> EPREEAGALGPAWDESQLRSYSFPTRPIPRLSQSDPR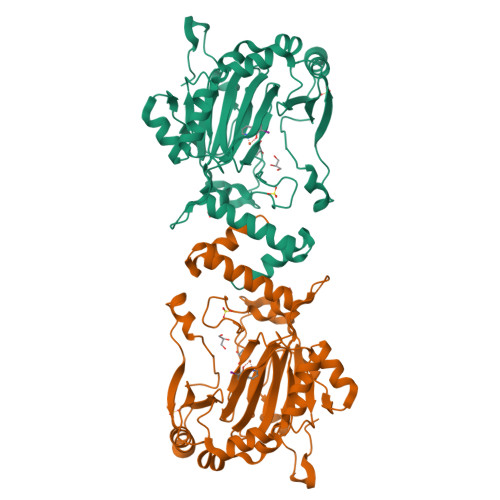AEELIENEEPVVLTDTNLVYPALKWDLEYLQENIGNGDFSVYSASTHKFLYYDEKKMANFQNFKPRSNREEMKFHEFVEKLQDIQQRGGEERLYLQQTLNDTVGRKIVMDFLGFNWNWINKQQGKRGWGQLTSNLLLIGMEGNVTPAHYDEQQNFFAQIKGYKRCILFPPDQFECLYPYPVHHPCDRQSQVDFDNPDYERFPNFQNVVGYETVVGPGDVLYIPMYWWHHIESLLNGGITITVNFWYKGAPTPKRIEYPLKAHQKVAIMRNIEKMLGEALGNPQEVGPLLNTMIKGRYN3-LAURYLAMIDO-N,N'-DIMETHYLPROPYLAMINOXYDE 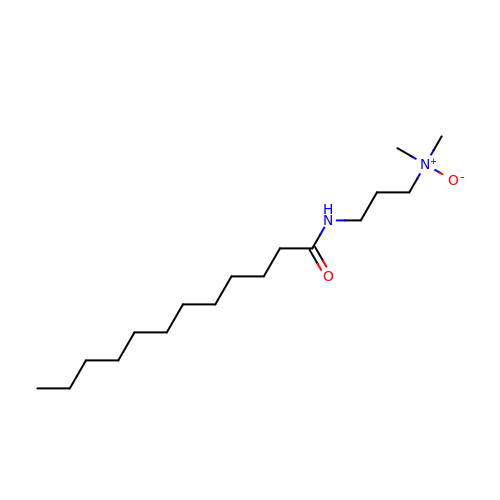| C17 H36 N2 O2 | JNGWKQJZIUZUPR-UHFFFAOYSA-N1-(biphenyl-3-yl)-3-hydroxypyridin-4(1H)-one 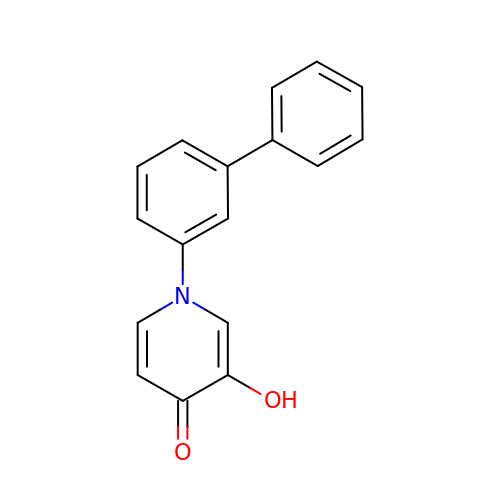| C17 H13 N O2 | IAMQYYMWXQPFDC-UHFFFAOYSA-N>PMTLGYWNIRGLAHSIRLLLEYTDSSYEEKKYTMGDAPDYDRSQWLNEKFKLGLDFPNLPYLIDGTHKITQSNAILRYIARKHNLCGESEKEQIREDILENQFMDSRMQLAKLCYDPDFEKLKPEYLQALPEMLKLYSQFLGKQPWFLGDKITFVDFIAYDVLERNQVFEPSCLDAFPNLKDFISRFEGLEKISAYMKSSRFLPRPVFTKMAVWGNK[2x];>[2x]SCESSMVLGYWDIRGLAHAIRLLLEFTDTSYEEKRYTCGEAPDY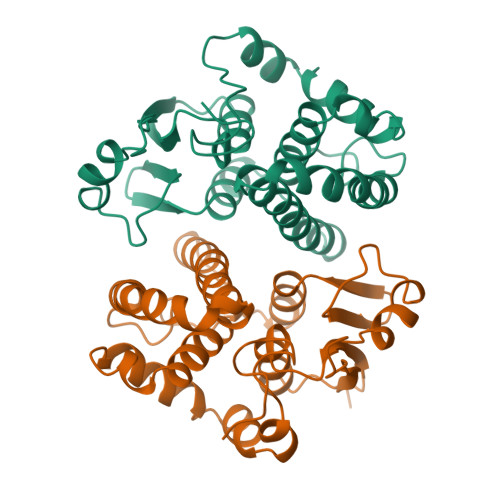DRSQWLDVKFKLDLDFPNLPYLLDGKNKITQSNAILRYIARKHNMCGETEEEKIRVDIIENQVMDFRTQLIRLCYSSDHEKLKPQYLEELPGQLKQFSMFLGKFSWFAGEKLTFVDFLTYDILDQNRIFDPKCLDEFPNLKAFMCRFEALEKIAAYLQSDQFCKMPINNKMAQWGNKPVC>[2x]METVAAIKTLIQQLAQSTDQFGRAEINDALRELQYSLETPFDTVMRMSLDTCQVAVARIGSDLGLFKHLSQCASPQSAEELADHLGCGRELMSRLLRYMASVRMVQQTDDIKYISSNITQTLAVPGLEAGMRHAFENLWPVLMALPDFLAERKYPDIVDAKDTAFQ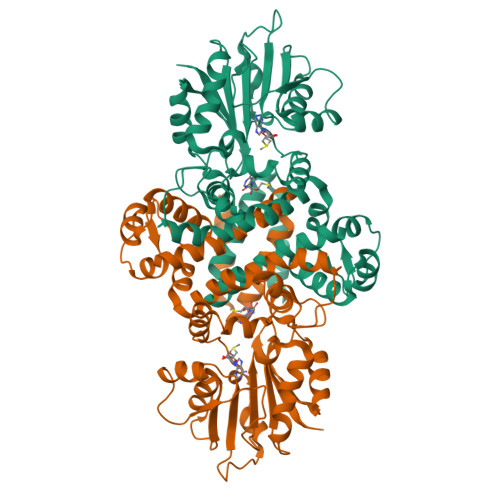KAFNTDQDCFHWLATQPTRIANFKVLLTDERTPNFLSTFPLEKELGSWSAEPEKALFVDIGGGMGHACIRLREKYPNQPGRVILQDLPPVLQAAQATLPLSGIESMPHNFHTPQPVQGAKFYFLRLILRDFPDHQALEILQNIVPAMDAESRIVIDDGVPPEKGARWAETGTDICIMSALGSKERTQRQWEELAAKAGLQLQALYQYTWPVVNAAMVFSLQ> GTRPRLKNVDRSTAQQLAVTVGNVTVIITDFK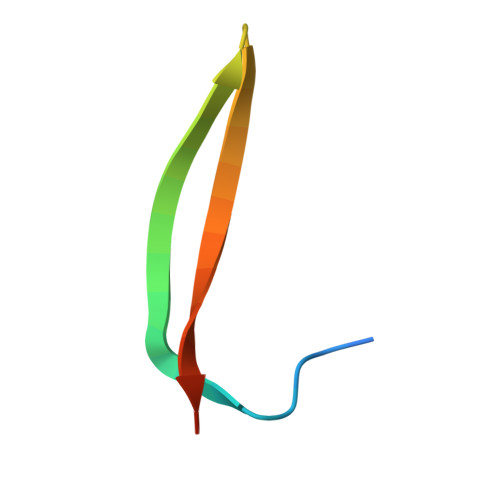EKTRS>GMKEDT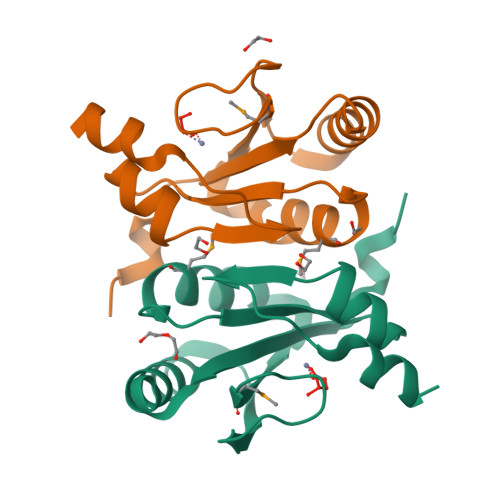IEIAGFHAHVYFDAASRDVAARVREGLGARFEVQLGRWFDKPIGPHPKGMYQVAFLPNQFDKVVPWLMLNREGLDILVHPETGDAVSDHAVYSLWLGAALALNIEFLRQLSSTSSN[2x]Here, we provide direct physiological, biochemical, and structural evidence for the anaerobic removal of iron from heme by HmuS, a membrane-bound, NADH-dependent de-chelatase that deconstructs heme to protoporphyrin IX (PPIX) and Fe(II). Phenotypic analyses of B. theta and its transposon insertion mutants demonstrate that HmuS, a large (1469 residues,163 kDa), multidomain membrane protein, is required for using heme as an iron source. HmuS de-chelatase shares the overall 6-domain architecture of these class I chelatases, including the N-terminal “head” (domain I) and “neck” (domain II) domains, followed by domains III–VI, which collectively form the body. The proposed structure-based mechanism for iron removal by HmuS is chemically analogous to the chelatases in both unrelated heme biosynthetic pathways and homologous enzymes in the biosynthetic pathways for chlorophyll and vitamin B12, although the reaction proceeds in the opposite direction.

Cryo-EM single particle analysis was used to determine two related structures of HmuS, each at a global resolution of 2.6 Å. With the exception of a disordered N-terminal domain in the second structure, they are highly similar. Thus, with the exception of the N-terminal domain, the structural description below applies to both structures. In this context, density for the head domain in the initial single particle map was relatively well ordered, but significantly weaker than the rest of the structure. Notably, the ordered structure retains strong density for the heme group at the interface of the head and neck domains. In contrast, heme density is absent in the disordered structure. These two structural snapshots are consistent with a mobile head domain in the absence of heme, which adopts an ordered conformation when heme is bound at the subunit interface. His-538 in the first motif and His-1209 in the second extend toward each other, directly across the middle of the putative active site, where they coordinate a strong spherical density, which we have modeled as a sodium cation due to the inclusion of NaCl in the buffer (EV4 and EV5). The flexible hinge connecting the head domain to the neck and the proximity of the MRI suggest that ferric heme can access a binding site at the head/neck interface, possibly fed by the MRI.

> MKKKSKIILGGCIVVAALIGLSVWNTWFSATKIAFVNFQTIQQGSISKANDNSFIKLSEVSLDNLDRLTSYDMVFINGMGLRIVEEQRQQIQQAADKGIPVYTSMATNPANNICNLDSIQQNLIRGYLSNGGKTNYRNMLNYIRKAIDGKASAVPEVEDPIERPSDMLYHAGISNPDDEQEFLTVADYEKFMQENNLYKEGARKIMITGQMADATDLIKALENAGYNVYPVQSMTRFMSFIEEVQPDAVINMAHGRMGDKMVDYLKARNILLFAPLTINSLVDEWENDPMGMSGGFMSQSIVTPEIDGAIRPFALFAQYEDKEGLRHSYAVPERLKTFVSTIDNYLNLKTKPNFEKKVAIYYYKGPGQNALTAAGMEVVPSLYNLLLRMKQEGYNISGLPANAQELGKMIQAQGAVFNAYAEGAFNDFMQNGHPELITKEQYESWVKESLRPEKYQEVVDAFGEFPGNYMVTPDGKLGIARLQFGNVVLLPQNAAGSGDNSFQVVHGTDMAPPHTYIASYLWMQHGFKADALIHFGTHGSLEFTPRKQVALCSNDWPDRLVGAVPHYYLYSIGNVGEGMMAKRRSYATLQSYLTPPFLESSVRGIYRELMEKIKIYNNSQKANKDQESLAVKTLTVKMGIHRDLGLDSMANKPYTEDEIARVENFAEELATEKITGQLYTMGVPYEPERITSSVYAMATEPIAYSLFALDKQRGKATESAEKHRSVFTQQYLMPARLLVERLMANPSLATDELICHTAGITPQELAKARQIEAERNAPKGMMAMMMAAAAKKDQADNEPSGNGHPASAKMEKGPHGKMPAGMKEAMKKMGANMDPEKAMEMAKSMGASPEALKKMEASMKANKDTSTDASGKPAMAGKTEKPQGMSAMMAAMGKAPKEYSKEEVEFALAVAEVERTIKNVGNYKNALLTSPEEELSSLMNALKGGYTAPTPGGDPIANPNTLPTGRNMYAINAEATPTESAWEKGIALAKQTIDRYKQRHNDSIPRKVSYTLWSSEFIETGGATIAQVLYMLGVEPVRDAFGRVSDLKLIPSTELGRPRIDVVVQTSGQLRDLAASRLFLINRAVEMAAAAKDDKYENQVASSVIEAERVLTEKGLSPKDAREISTFRVFGGANGMYGTGIQEMVESGDRWENESEIADTYLNNMGAYYGSEKNWEVFQKFAFEAALTRTDVVVQPRQSNTWGALSLDHVYEFMGGMNLAVRNVTGKDPDAYLSDYRNRNHMKMQELKEAVGVESRTTILNPTYIKEKMKGGASSASEFAEVITNTYGWNVMKPAAIDKELWDNIYNVYVKDELNLGVKQYFEQQNPAALEEMTAVMLESARKGLWQASEEQVAELSKLHTEIVNTYRPSCSGFVCDNAKLRDFIASKADAQTATQYKENISKIREAKASGSNKGVVMKKEEMNQTAENQTNTLSNVAVGIAVIIVILALILFVRKRRKSSQM>[3x]MELMMAIGYLGLALVLGSLVAKIAEKLKIPDIPLLLLLGLIIGPFLQIIPSDSAMEIFEYAGPIGLIFILLGGAFTMRISLLKRVIKTVVRLDTITFLITLLISGFIFNMVLNLPYTSPVGYLFGAITAATDPATLIPVFSRVRTNPEVAITLEAESIFNDPLGIVSTSVILGLFGLFSSSNPLIDLITLAGGAIVVGLLLAKIYEKIIIHCDFHEYVAPLVLGGAMLLLYVGDDLLPSICGYGFSGYMAVAIMGLYLGDALFRADDIDYKYIVSFCDDLSLLARVFIFVFLGACIKLSMLENYFIPGLLVALGSIFLARPLGVFLGLIGSKHSFKEKLYFALEGPRGVVPAALAVTVGIEILKNADKIPASITKYITPTDIAGTIIIGTFMTILLSVILEASWAGMLALKLLGEYKPKYKEESHH;> MELMMAIGYLGLALVLGSLVAKIAEKLKIPDIPLLLLLGLIIGPFLQIIPSDSAMEIFEYAGPIGLIFILLGGAFTMRISLLKRVIKTVVRLDTITFLITLLISGFIFNMVLNLPYTSPVGYLFGAITAATDPATLIPVFSRVRTNPEVAITLEAESIFNDPLGIVSTSVILGLFGLFSSSNPLIDLITLAGGAIVVGLLLAKIYEKIIIHCDFHEYVAPLVLGGAMLLLYVGDDLLPSICGYGFSGYMAVAIMGLYLGDALFRADDIDYKYIVSFCDDLSLLARVFIFVFLGACIKLSMLENYFIPGLLVALGSIFLARPLGVFLGLIGSKHSFKEKLYFALEGPRGVVPAALAVTVGIEILKNAEKIPASITKYITPTDIAGTIIIGTFMTILLSVILEASWAGMLALKLLGEYKPKYKEESHH

MjNhaP1 has 13 transmembrane helices (TMH), referred to as H1-13. Unlike PaNhaP, MjNhaP1 is not cooperative at any pH tested. MjNhaP1 is inhibited by the Myc-His-Tag at pH 8 but not at pH 6.

asymmetric unit were refined to 3.5 Å resolution. Detailed views of the MjNhaP1 x-ray structure. Glu154 in H6 interacts with Thr76 in the interface helix H3. Arg320 forms an ion bridge with Glu156. Nevertheless, changing N160 to alanine renders MjNhaP1 inactive. closely resembles the x-ray structure of MjNhaP1 rather than that of EcNhaA. inward-open and the EM structure the outward-open state. inward-open with a sodium ion in the binding site.>TKAVHTKHAPAAIGPYSQGIIVNNMFYSSGQIPLTPSGEMVNGDIKEQTHQVFSNLKAVLEEAGAS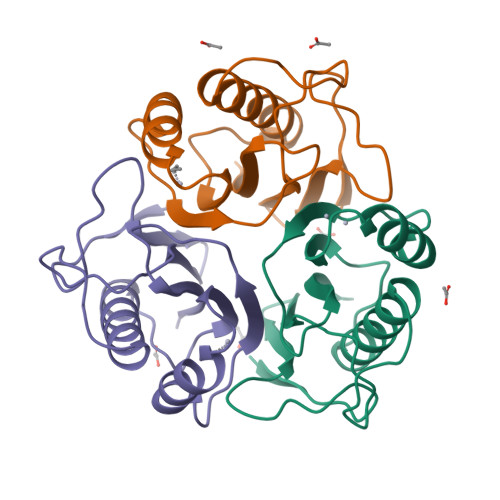FETVVKATVFIADMEQFAEVNEVYGQYFDTHKPARSCVEVARLPKDALVEIEVIALVK[3x]> MGVSPAAPASGIRRPCYLVLSSHDFRTPRRANIHFITDQLALRGTTRFFSLRYSRLSRMKGDMRLPLDDTANTVVSHNGVDCYLWRTTVHPFNTRRSWLRPVEDAMFRWYAAHPPKQLLDWMRESDVIVFESGIAVAFIELAKRVNPAAKLVYRASDGLSTINVASYIEREFDRVAPTLDVIALVSPAMAAEVVSRDNVFHVGHGVDHNLDQLGDPSPYAEGIHAVAVGSMLFDPEFFVVASKAFPQVTFHVIGSGMGRHPGYGDNVIVYGEMKHAQTIGYIKHARFGIAPYASEQVPVYLADSSMKLLQYDFFGLPAVCPNAVVGPYKSRFGYTPGNADSVIAAITQALEAPRVRYRQCLNWSDTTDRVLDP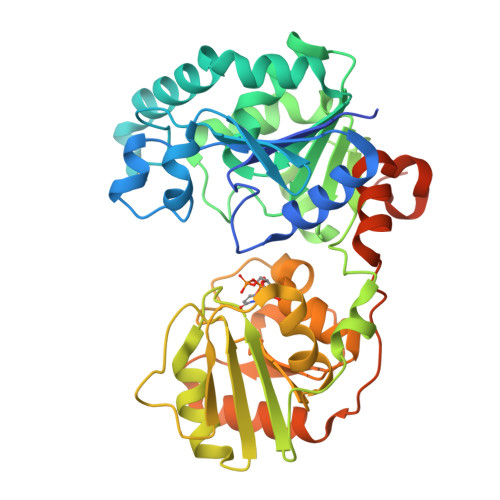RAYPETRLYPHPPTAAPQLSSEAALSHHHHHHH> GS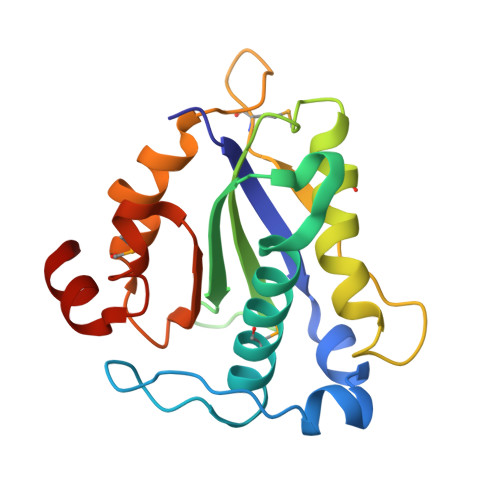ELFRGVLQVSSNVLDCANDNWWCSLLDLDTSDWEPLTHTNRLMAIYLSSVASKLDFTGGPLAGCLYFFQVECNKFEEGYHIHVVIGGPGLNPRNLTVCVEGLFNNVLYHLVTGNVKLKFLPGMTTKGKYFRDGEQFIENYLMKKIPLNVVWCVTNIDGYIDTCISATFRRGACHA> ADTIVAVELDSYPNTDIGDPNYPHIGIDIKSIRSKSTARWNMQTGKVGTVHIS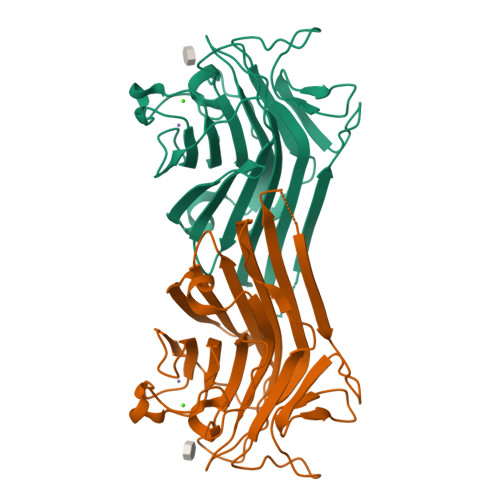YNSVAKRLSAVVSYSGSSSTTVSYDVDLNNVLPEWVRVGLSATTGLYKETNTILSWSFTSKLKTNSIADENSLHFSFHKFSQNPKDLILQGDAFTDSDGNLQLTKVSSSGDPQGNSVGRALFYAPVHIWEKSAVVASFDATFTFLIKSPDREPADGITFFIANTDTSIPSGSGGRLLGLFPDAN The amyloid β-peptide (Aβ), usually containing 40–42 amino acids, is derived from the β-amyloid precursor protein (APP) by subsequent proteolyses processed by β-site cleaving enzyme (BACE1) and γ-secretase. Based on the amyloid hypothesis, BACE1 is recognized as an important drug target since it is the rate-limited enzyme during the production of Aβ and initializes the cleavage of APP. Structurally, BACE1 belongs to the aspartyl protease family, and contains a bilobal structure forming by an N- and a C-terminal domains. Both N- and C-domains are formed by highly twisted β-sheet structures and each domain contributes an aspartic acid to the catalytic module of the enzyme.

Nitrile group was the optimal substitutent on indole, especially, when the nitrile group was introduce into the 6-position of indole (compound 25), the most potent analog was identified, which was nearly 23-fold more potent than compound 19 and >1,000-fold more potent than the fragment hit resulting from virtual screening (compound 4, IC50 > 100 µM). Ligand 25 is situated in a similar position as ligand 19 in the binding pocket of BACE1. The guanidine group again forms critical H-bonding interactions with the two catalytic residues Asp32 and Asp228. The substituted nitrile group forms a new hydrogen bond with Ser328, which may account for the improvement of its binding affinity. This subpocket located at the opposite of flap loop, which is under-explored in previous studies on the discovery of BACE1 inhibitors. The SAR study in the present work further demonstrates its value for future inhibitor design. The superimposition of structures of BACE1 in complex with compounds 19, 25 and the initial docked fragment are also shown.

> MGSSHHHHHHSAGENLYFQGTLPRETDEEPEEPGRRGSFVEMVDNLRGKSGQGYYVEMTVGSPPQTLNILVDTGSSNFAVGAAPHPFLHRYYQRQLSSTYRDLRKGVYVPYTQGAWAGELGTDLVSIPHGPNVTVRANIAAITESDKFFINGSNWEGILGLAYAEIARPDDSLEPFFDSLVKQTHVPNLFSLQLCGAGFPLNQSEVLASVGGSMIIGGIDHSLYTGSLWYTPIRREWYYEVIIVRVEINGQDLKMDCKEYNYDKSIVDSGTTNLRLPKKVFEAAVKSIKAASSTEKFPDGFWLGEQLVCWQAGTTPWNIFPVISLYLMGEVTNQSFRITILPQQYLRPVEDVATSQDDCYKFAISQSSTGTVMGAVIMEGFYVVFDRARKRIGFAVSACHVHDEFRTAAVEGPFVTLDMEDCGYNIPQTDEST> GWLAPEQQQ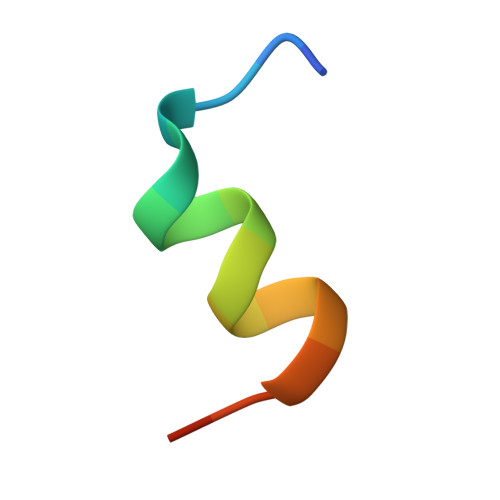RIYRGNAS>GPGSMALERTLSIIKPDAVAKNVIGQIYSRFENAGLKIVAARMAHLSRADAEKFYAVHAERPFFKDLVEFMISGP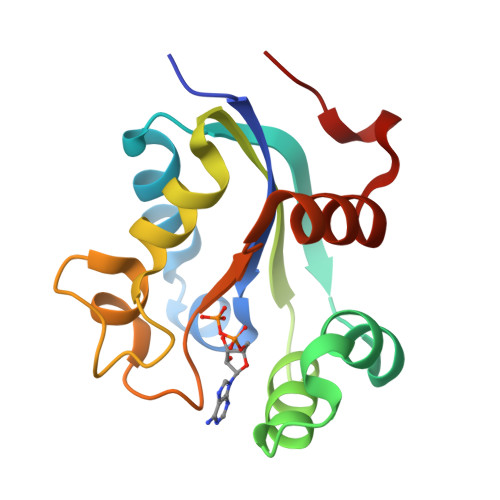VMIQVLEGEDAILKNRDLMGATDPKKAEKGTIRADFADSIDANAVHGSDAPETARVEIAFFFPEMNVYSR[2x]>[2x]TEKKYIVALDQGTTSSRAVVMDHDANIISVSQREFEQIYPKPGWVEHDPMEIWATQSSTLVEVLAKADISSDQIAAIGITNQRETTIVWEKETGKPIYNAIVWQCRRTAEICEHLKRDGLEDYIRSNTGLVIDPYFSGTKVKWILDHVEGSRERARRGELLFGTVDTWLIWKMTQGRVHVTDYTNASRTMLFNIHTLDWDDKMLEVLDIPREMLPEVRRSSEVYG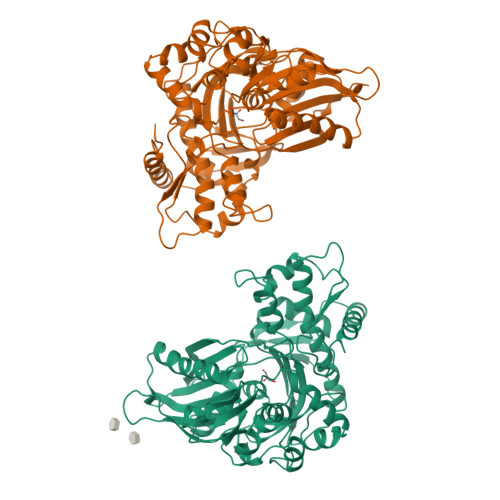QTNIGGKGGTRIPISGIAGDQQAALFGQLCVKEGMAKNTYGTGCFMLMNTGEKAVKSENGLLTTIACGPTGEVNYALEGAVFMAGASIQWLRDEMKLINDAYDSEYFATKVQNTNGVYVVPAFTGLGAPYWDPYARGAIFGLTRGVNANHIIRATLESIAYQTRDVLEAMQADSGIRLHALRVDGGAVANNFLMQFQSDILGTRVERPEVREVTALGAAYLAGLAVGFWQNLDELQEKAVIEREFRPGIETTERNYRYAGWKKAVKRAMAWEEHDE(2~{R},3~{S},4~{R},5~{R},6~{R})-5-azanyl-2-(hydroxymethyl)-6-(5-phenyl-4~{H}-1,2,4-triazol-3-yl)oxane-3,4-diol 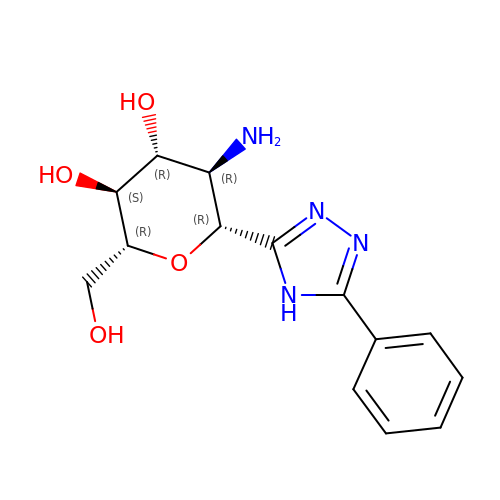| C14 H18 N4 O4 | RPVORBKHTZKTGY-LZQZFOIKSA-N>[2x]QDSTSDLIPAPPLSKVPLQQNFQDNQFHGKWYVVGLAGNGNLREDKDPLKMYATIYELKEDKSYNVTDVLFIDKKCHYLINTFVPGSQPGEFTLGSIKSTLGSTSRLVRVVSTNYNQHAMVFFKWVHQNREWFYITLYGRTKELTSELKENFIRFSKSLGLPENHIVFPVPIDQCIDGSAHHHHHH;>ASWSHPQFEKGAELPVQRWWHKGALYRIGDLQAFVGRDAGGIAGLKSHLEYLSTLKVKGLVLGPIHKNQKDEINETDLKQINPTLGSQEDFKDLLQSAKKKS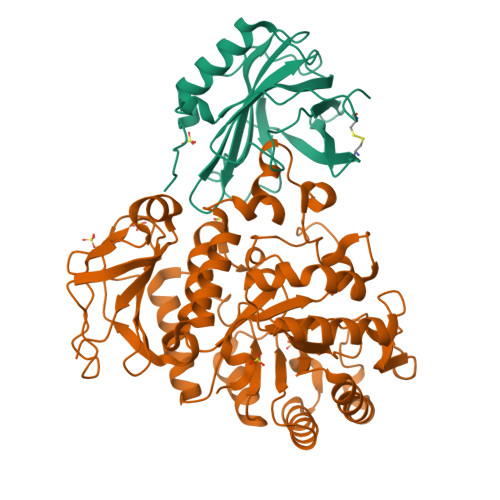IHIILDLTPNYQGQNAWFLPAQADIVATKMKEALSSWLQDGVDGFQFRDVGKLMNAPLYLAEWQNITKNLSEDRLLIAGTESSDLQQIVNILESTSDLLLTSSYLSNSTFTGERTESLVTRFLNATGSQWCSWSVSQAGLLADFIPDHLLRLYQLLLFTLPGTPVFSYGDELGLQGALPGQPAKAPLMPWNESSIFHIPRPVSLNMTVKGQNEDPGSLLTQFRRLSDLRGKERSLLHGDFHALSSSPDLFSYIRHWDQNERYLVVLNFRDSGRSARLGASNLPAGISLPASAKLLLSTDSARQSREEDTSLKLENLSLNPYEGLLLQFPFVA[2x]>MADLFNKHLKKATNRTKEKLLEGIGKAKATQDEVFDQHAANLNKQSKSCEKLHKDVKNYSSALRTLLSAEKQLRDTIRDAYEPEWPDREHLTAIFDNLDIQTNELEKTVCDDLPQTVTQYVNQFPDLKKKIEKRGRKLVDYDSAKNSFNSVKASSKKDNDPKLAKATMELQAAEQMYTEMNNELLEILPAVFDSRITFFVDTLQTLFNANSVYQ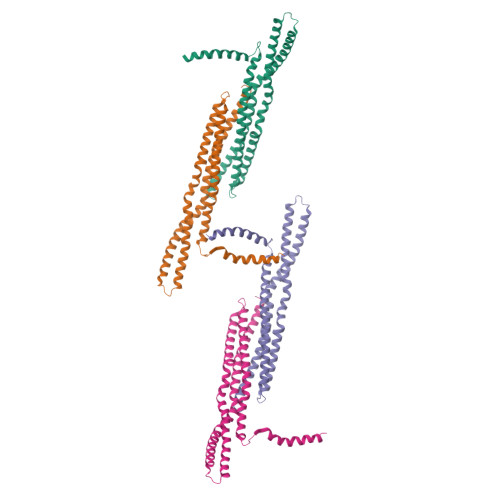TDASKFHKQIVMQLDKLGESMDYL[4x]> 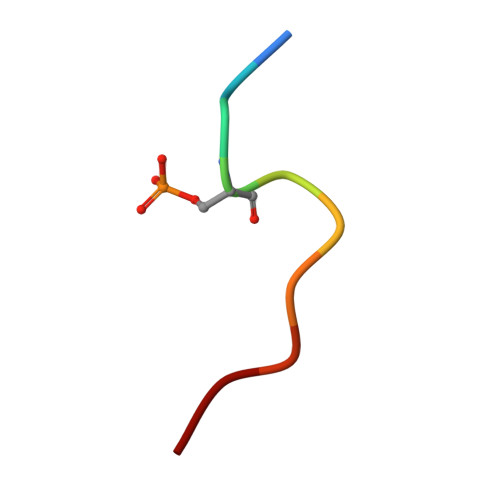ERESEFDIED>[2x]MKYFSFSLSFPKITIFLFSFVLVASANHAHESFLECLTTRISKSNSTSTPESIIYTKDNPSYS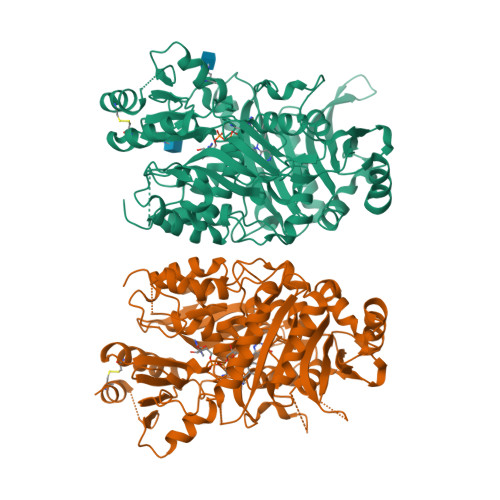TILNSTSLNPRFFPSSARYPLLIVTPLHASHVQATVHCAKKHGIQIRIRSGGHDYEGLSYMSNVTFAIVDLRNLSSIDVDVKRKSAWVQSGATLGELHYWIAKKSQNLAFPGVVGHTVGIGGMLGAGGYGYSSRKYGLSADNILDAQLIDVRGRILNRKSMGEDLFWAIRGGGAGSFGIVLAWKVRLVDVPSKVTVFTAIRDWDNNATKKFIHRYQRRIAKVDKDLTIIVRFLTASITDEKGSKKIQISTFITATYHGSQDRLLSLMEKEFPELGLLAKECAEGAWVQSILYFNLLTNSKSLDVLLNRTLNFEWRAFKIKSDYLKKPIPDQVLENLLVKLYEEDIGETFVEFFPYGGKLDEISESEIPCPHRAGNLYNLRYMVLWKEGQNATAVNKHLSWIRRAYNYMTPYVSKNPRGAFLNFRDLDIGTNPNENEINGAYNYIKQASNWGTKYFKNNFYKLIYVKTIVDPTNFFTYEQSIPSLLPH>MATHHTLWMGLALLGVLGDLQAAPEAQVSVQPNFQQDKFLGRWFSAGLASNSSFLREKKAALSMAKSVVAPATDGGLNLTSTFLRKN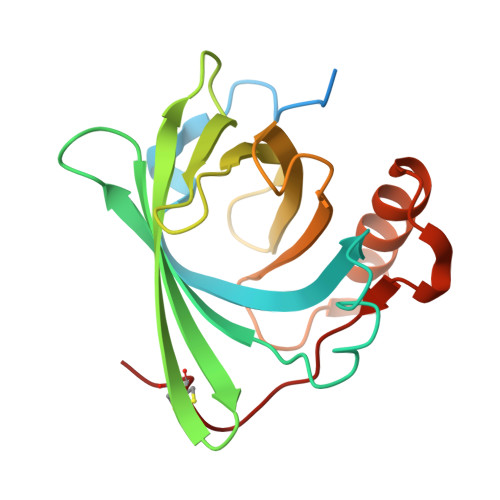QCETRTMLLQPAGSLGSYSYRSPHWGSTYSVSVVETDYDQYALLYSQGSKGPGEDFRMATLYSRTQTPRAELKEKFTAFCKAQGFTEDTIVFLPQTDKCMTEQ[2x]FARNESYL | C15 H26 | 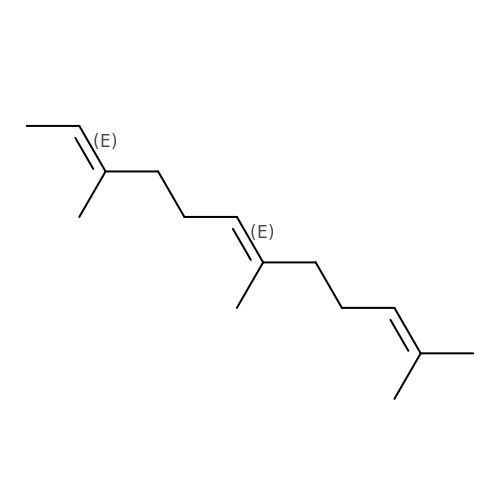JXBSHSBNOVLGHF-BUJBXKITSA-N> GPLGSPEFPGRLEMEPDFYCVKWIPWKGEQTPIITQST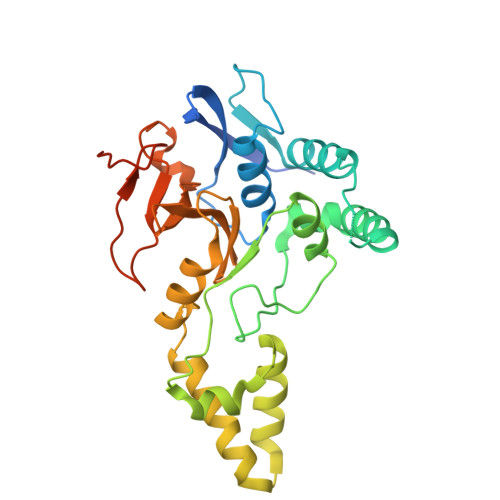NGPCPLLAIMNILFLQWKVKLPPQKEVITSDELMAHLGNCLLSIKPQEKSEGLQLNFQQNVDDAMTVLPKLATGLDVNVRFTGVSDFEYTPECSVFDLLGIPLYHGWLVDPQSPEAVRAVGKLSYNQLVERIITCKHSSDTNLVTEGLIAEQFLETTAAQLTYHGLCELTAAAKEGELSVFFRNNHFSTMTKHKSHLYLLVDDQGFLQEEQVVWESLHNVDGDSCFCDSDFHLSHSLGKGPGAEGGSGSPE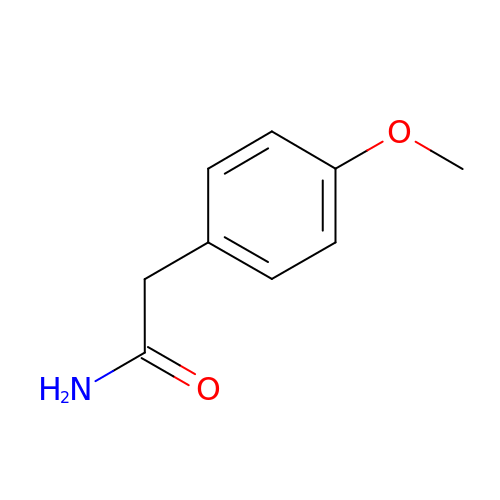2-(4-METHOXYPHENYL)ACETAMIDE | C9 H11 N O2 | OLKQIWCQICCYQS-UHFFFAOYSA-N>MNPAAEAEFNILLATDSYKVTHYKQYPPNTSKVYSYFECREKKTENSKLRKVKYEETVFYGLQYILNKYLKGKVVTKEKIQEAKDVYKEHFQDDVFNEKGWNYILEKYDGHLPIEIKAVPEGFVIPRGNVLFTVENTDPECYWLTNWIETILVQSWYPITVATNSREQKKILAKYLLETSGNLDGLEYKLHDFGYRGVSSQETAGIGASAHLVNFKGTDTVAGLALIKKYYGTKDPVPGYSVPAAEHSTITAWGKDHEKDAFEHIVTQFSSVPVSVVSDSYDIYNACEKIWGEDLRHLIVSRSTQAP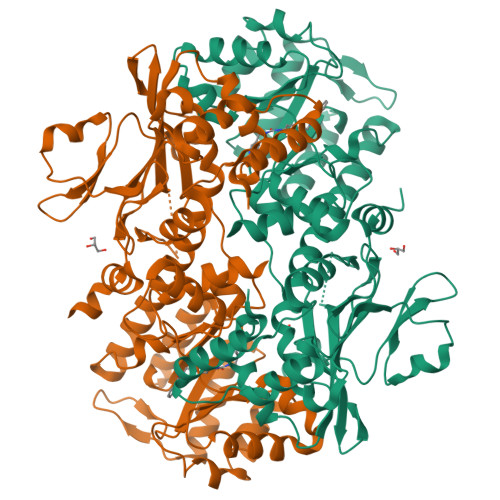LIIRPDSGNPLDTVLKVLEILGKKFPVTENSKGYKLLPPYLRVIQGDGVDINTLQEIVEGMKQKMWSIENIAFGSGGGLLQKLTRDLLNCSFKCSYVVTNGLGINVFKDPVADPNKRSKKGRLSLHRTPAGNFVTLEEGKGDLEEYGQDLLHTVFKNGKVTKSYSFDEIRKNAQLNIELEAAHHLEHHHHHHHH[4x]>[2x]MSIFPKISLRPEVENYLKEGFMNKEIVTALGKQEAERKFETLLKHLSHPPSFTTVRVNTHLASVQHVKNLLLDELQKQFNGLSVPILQHPDLQDVLLIPVIGPRKNIKKQQCEAIVGAQCGNAVLRGAHVYAPGIVSASQFMKAGDVISVYSDIKGKCKKGAKEFDGTKVFLGNGISELSRKEIFSGLPELKGMGIRM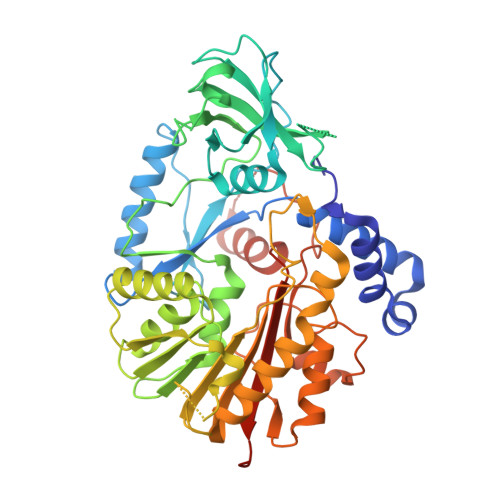TEPVYLSPSFDSVLPRYLFLQNLPSALVSHVLNPQPGEKILDLCAAPGGKTTHIAALMHDQGEVIALDKIFNKVEKIKQNALLLGLNSIRAFCFDGTKAVKLDMVEDTEGEPPFLPESFDRILLDAPCSGMGQRPNMACTWSVKEVASYQPLQRKLFTAAVQLLKPEGVLVYSTCTITLAENEEQVAWALTKFPCLQLQPQEPQIGGEGMRGAGLSCEQLKQLQRFDPSAVPLPDTDMDSLREARREDMLRLANKDSIGFFIAKFVKCKSTLEHHHHHH N-({4-[(6aR)-3-amino-1-oxo-1,2,5,6,6a,7-hexahydroimidazo[1,5-f]pteridin-8(9H)-yl]phenyl}carbonyl)-L-glutamic 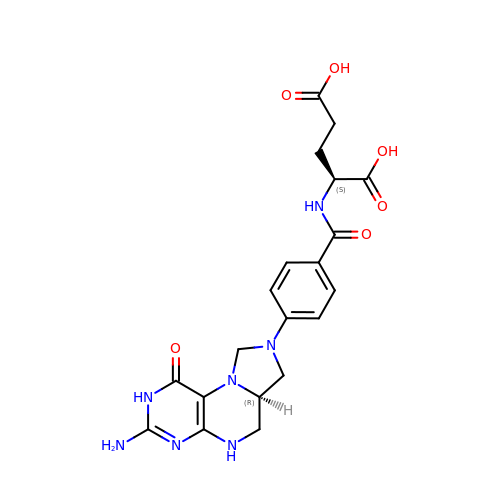acid | C20 H23 N7 O6 | QYNUQALWYRSVHF-OLZOCXBDSA-N>MSKLIVPQWPQPKGVAACSSTRIGGVSLPPYDSLNLGAHCGDNPDHVEENRKRLFAAGNLPSKPVWLEQVHGKDVLKLTGEPYASKRADASYSNTPGTVCAVMTADALPVLFCNRAGTEVAAAHAGWRGLCAGVLEETVSCFADN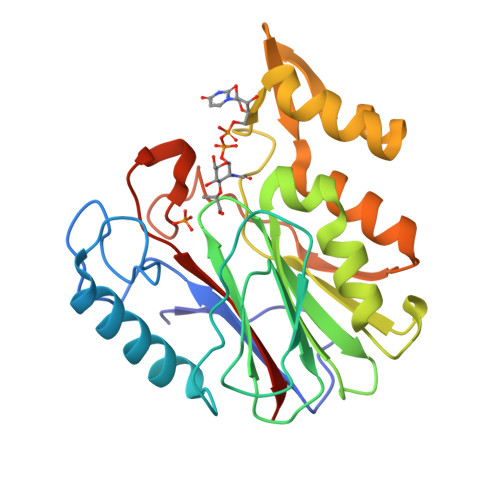PENILAWLGPAIGPRAFEVGGEVREAFMAVDAKASAAFIQHGDKYLADIYQLARQRLANVGVEQIFGGDRCTYTENETFFSYRRDKTTGRMASFIWLILEHHHHHH[4x]>[4x]QAEEWYFGKITRRESERLLLNPENPRGTFL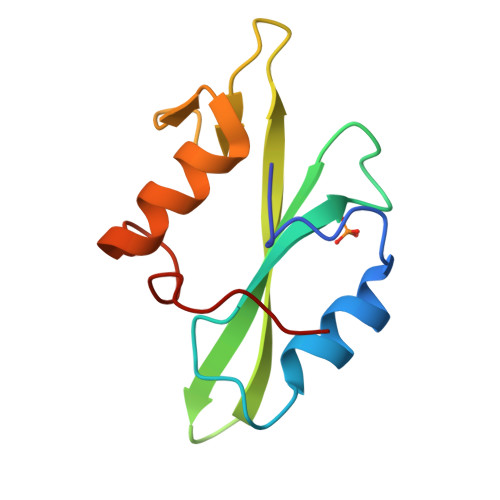VRESETTKGAYCLSVSDFDNAKGLNVKHYKIRKLDSGGFYITSRTQFSSLQQLVAYYSKHADGLCHRLTNVCPT> MAEQVALSRTQVCGILREELFQGDAFHQSDTHIFIIMGASGDLAKKKIYPTIWWLFRDGLLPENTFIVGYARSRLTVADIRKQSEPFFK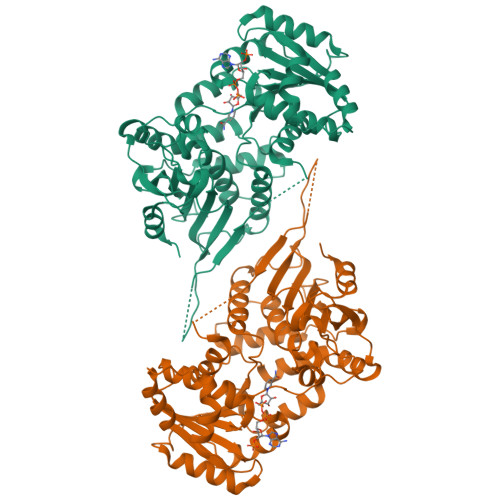ATPEEKLKLEDFFARNSYVAGQYDDAASYQRLNSHMNALHLGSQANRLFYLALPPTVYEAVTKNIHESCMSQIGWNRIIVEKPFGRDLQSSDRLSNHISSLFREDQIYRIDHYLGKEMVQNLMVLRFANRIFGPIWNRDNIACVILTFKEPFGTEGRGGYFDEFGIIRDVMQNHLLQMLCLVAMEKPASTNSDDVRDEKVKVLKCISEVQANNVVLGQYVGNPDGEGEATKGYLDDPTVPRGSTTATFAAVVLYVENERWDGVPFILRCGKALNERKAEVRLQFHDVAGDIFHQQCKRNELVIHVQPNEAVYTKMMTKKPGMFFNPEESELDLTYGNRYKNVKLPDAYERLILDVFCGSQMHFVRSDELREAWRIFTPLLHQIELEKPKPIPYIYGSRGPTEADELMKRVGFQYEGTYKWVNPHKL>[2x]MGMAEVSSKRRKRTKTDIGCQSSAI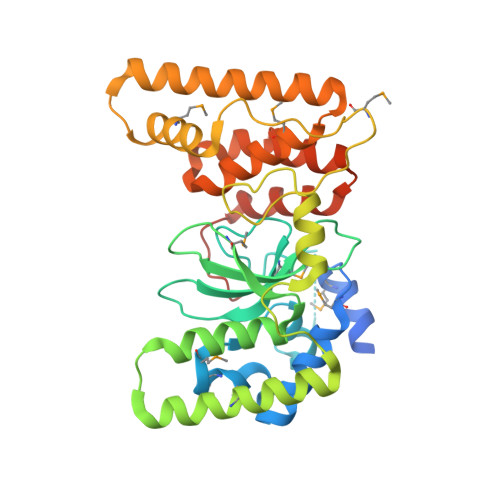KKIKEMFDAVMPEDFYDFWAFCEELNPKNPEDALMDTMGLQLVGPYDVLTGKLDGLSESSYHLHWRYYYDPPEFMTVIRGNEDQGFHIGYYRDEPQALPVFVASNKAKVSCEMSVIGENLFSALNTCITENLKKIKDKSQQSSLKKMQTSLITKAKELQYSLATTTPAIKARNKKVNSKTLHKAGIVVPVNAMDVGYRPLTVTDAELKKMLKTITESENKSAKDKASDELQELLTFVQFANDEGDYGMGLELGLDLFCFGSKQFHNTILQLLPLAYQLLGREKYAKIIQEHLENRDREKLSEASKHHHHHH> MGSDKIHHHHHHMNNQEKNMLGFNQDEYLTSAREIIAARQKAEQVADEIYQAGFSSLFFASVGGSLAPMMAINEFAKELTTLPVYVEQAAELIHKGNKRLNKDSVVITLSKSGDTKESVAIAEWCKAQGIRVVAITKNADSPLAQAATWHIPMRHKNGVEYEYMLLYWLFFRVLSRNNEFASYDRFASQLEILPANLLKAKQKFDPQADAIASRYHNSDYMMWVGGAEMWGEVYLFSMCILEEMQWKRTRPVSSAEFFHGALELLEKDVPLILVKGEGKCRALDERVERFASKITDNLVVIDPKAYALDGIDDE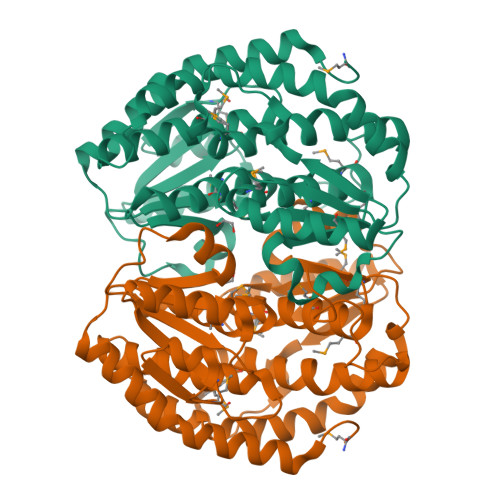FRWIMAPCVVSTLLVDRLAAHFEKYTGHSLDIRRYYRQFDY3-hydroxy-2-iminopropanoic acid | C3 H5 N O3 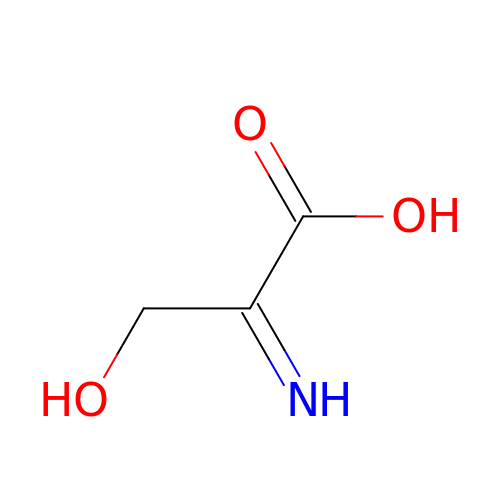| MUHXUPVPXJXCGV-DUXPYHPUSA-N> MRNKIFISHATPEDDDFTRWLSLKLIGLGYEVWCDILFLDKGVDFWSTIEKEIRENTCKFLIVSSTAGNKREGVLKELAVATKVKKHLQDDMFIIPLAIDENLSYDDINIEIVRLNAIDFKKSWAKGLQDLLDAFEKQNVPKKPPDHSKSNLLYQQIFLHDKQAIEKEETYDSNWFPIISFPNELRFHRYDWRLPKQFDVRTLAFPAIRYKEYLCTFAWEYDFIHQLPKTETYNGQESIRISTSDILSGRYDTDFIRNYECQRLIVQLINKAFELRMKDKNVREYQMSKTFAYWIEKGKLEKDKFEKIKLVGKQKNKYWHFGISAAGKLYPSPVLMVSSHIIFTMDGINLIKSKSIQHS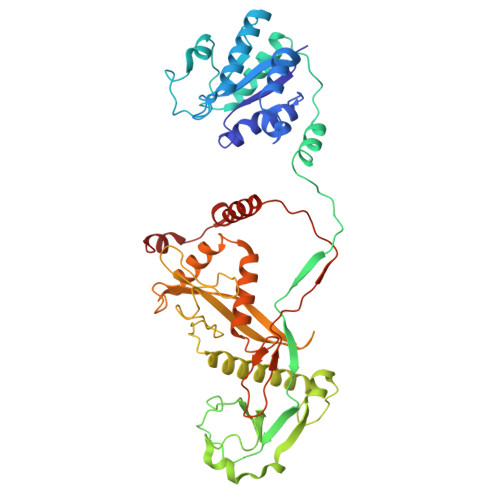SRRKQGKNWWNDKWREKLLAFIRFLSDDQNAIYLNVGSEEKILISNKPLKFFGKMSYVTPSEVTLEEESVLADINNFEEDTEDLDELEDIE>MTSITPVTLANCEDEPIHVPGAIQPHGALVTLRADGMVLAASENIQALLGFVASPGSYLTQEQVGPEVLRMLEEGLTGNGPWSNSVETRIGEHLFDVIGHSYKEVFYLEFEIRTADTLSITSFTLNAQRIIAQVQLHNDTASLLSNVTDELRRMTGYDRVMAYRFRHDDSGEVVAESRREDLESYLGQRYPASDIPAQARRLYIQNPIRLIADVAYTPMRVFPALNPETNESFDLSYSVLRSVSPIHCEYLTNMGVRASMSISIVVGGKLWGLFSCHHMSPKLIPYPVRMSFQIFSQVCSAIVERLEQGRIAELLRVSTERRLALARRARDADDLFGALAHPDDGIAALIPCDGALVMLGGRTLSIRGDFERQAGNVLQRLQRDPERDIYHTDNWPQPSEDSPDGGDCCGVLAIRFHRQESGWIFWFRHEEVHRIRWGGKPEKLLTIGPSGPRLTPRGSFEAWEEVVRGHSTPWSETDLAIAEKLRLDLMELCLNHAAEVDRMRQRLIAVLGHDLRNPLQSISMAAALLSSSDTRTTELRQHISASSSRMERLVSQILDMSRLQSGIGLTVNPVDTDVSQLVRQIVCETDVAYPGLVIEIAIDPQVRAVVDPDRYAQVAANLLSNARHHGLPGRPVLVTLTRQGDEVCLSVL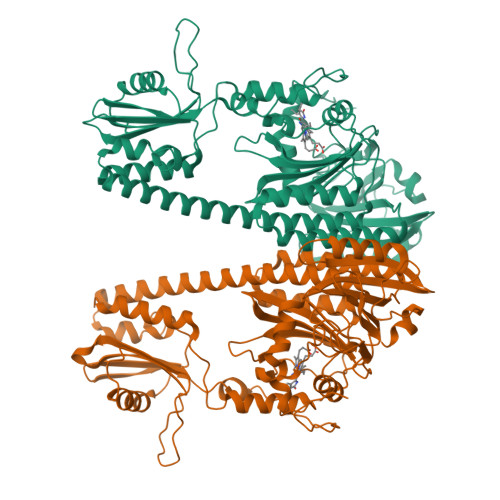NETSGLSEAQLANLFEPFKRESADNQRNRNGLGIGLYISQAIAQAHQGRIDVDCRDDVITFCLRLPVRQAETGSSSLEHHHHHH[2x]>[2x]SNAMRLTDQKRESIVQAAIAEFGDRGFEITSMDRIAARAEVSKRTVYNHFPSKEELFAEMLQRLWNCAPPQSEVVYRPLVSLREQLLELLWGKMRNL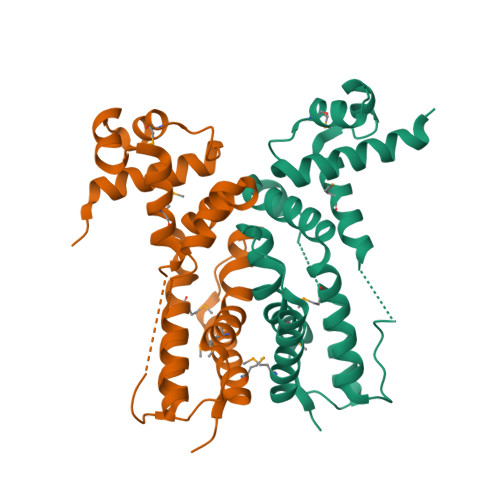TDSSFLDLARVVVGATIHSPERAQVWLARINEREETFSAWIRAAQKDGRLKPVDPGFAATQMHALLKSFAFWPQVTFNAALLTPQEQSNVVESALNMFLGWYEIPG>[4x]MKLLKILSLVCLSISIGACAEHSMSRAKTSTI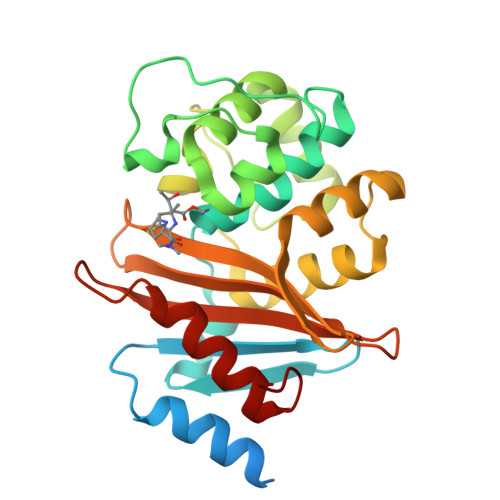PQVNNSIIDQNVQALFNEISADAVFVTYDGQNIKKYGTHLDRAKTAYIPASTFKIANALIGLENHKATSTEIFKWDGKPRFFKAWDKDFTLGEAMQASTVPVYQELARRIGPSLMQSELQRIGYGNMQIGTEVDQFWLKGPLTITPIQEVKFVYDLAQGQLPFKPEVQQQVKEMLYVERRGENRLYAKSGWGMAVDPQVGWYVGFVEKADGQVVAFALNMQMKAGDDIALRKQLSLDVLDKLGVFHYL> SNAMSEWSRIAVEFGEQQLNLTELEDFARELAYEGLDPALIIKKLKETGGDDWVKDTKFIIVFALTRGNKIVKASGKMSNSGSKRLMALQEKYGLVERAETRLSITPVRVAQSLPTWTCAAAAALKEYLPVGPAVMNLKVENYPPEMMCMAFGSLIPTAGVSEATTKTLMEAYSLWQDAFTKTINVKMRGASKTEVYNSFRDPLHAAVNSVFFPNDVRVKWLKAKGILGPDGVPSRAAEVAAAAY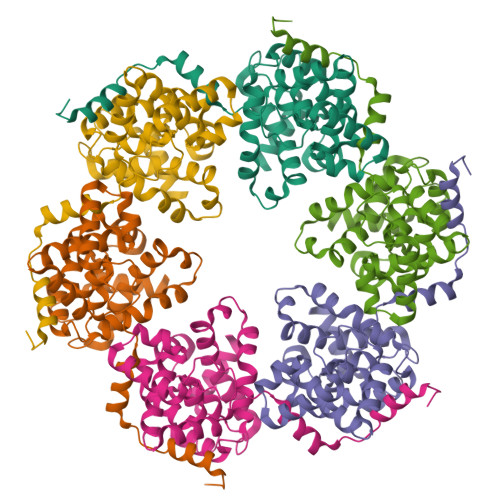RNL>MNPELEEWIRRAKEVAKEVEKVAQRAEEEGNPDLRDSAKELRRAVEEAIEEAKKQGNPELVEWVARAAKVAAEVIKVAIQAEKEGNRDLFRAALELVRAVIEAIEEAVKQGNPELVEWVARAAKVAAEVIKVAIQAEKEGNRDLFRAALELVRAVIEAIEEAVKQGNPELVERVARL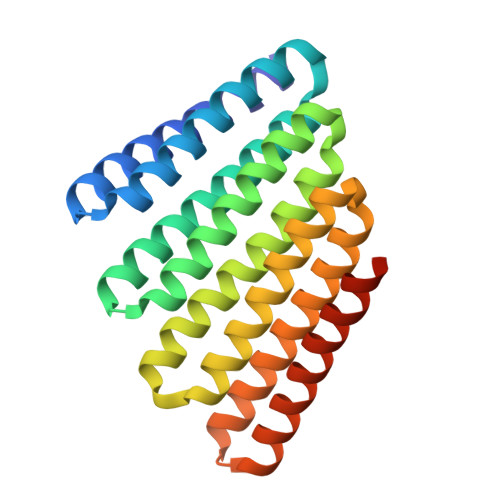AKKAAELIKRAIRAEKEGNRDERREALERVREVIERIEELVRQGGWLEHHHHHH[2x]>[2x]RIKKISIEGNIAA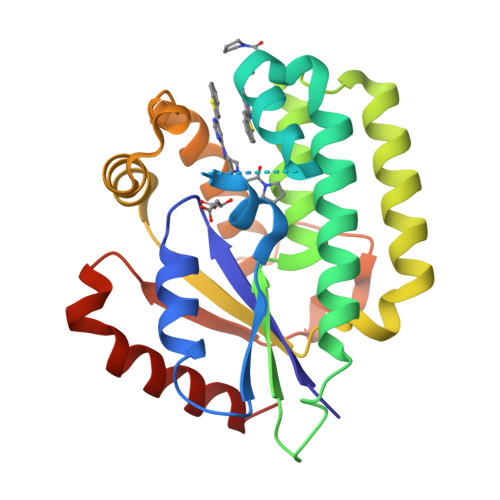GKSTFVNILKQLCEDWEVVPEPVARWCNVQSTQDEFEELTMSQKNGGNVLQMMYEKPERWSFTFQTYACLSRIRAQLASLNGKLKDAEKPVLFFERSVYSDRYIFASNLYESECMNETEWTIYQDWHDWMNNQFGQSLELDGIIYLQATPETCLHRIYLRGRNEEQGIPLEYLEKLHYKHESWLLHRTLKTNFDYLQEVPILTLDVNEDFKDKYESLVEKVKEFLSTL> MLADKESLIEALKLALSTEYNVKRNF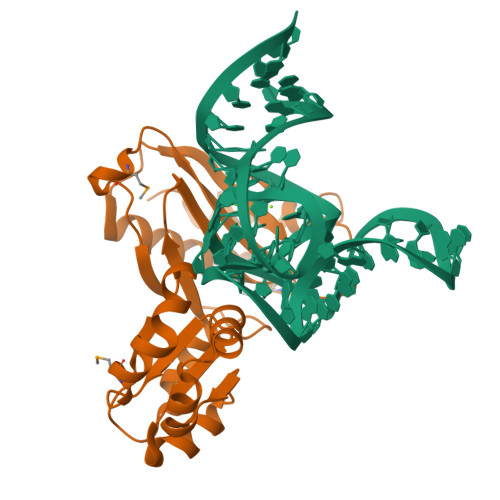TQSVEIILTFKGIDMKKGDLKLREIVPLPKQPSKAKRVLVVPSSEQLEYAKKASPKVVITREELQKLQGQKRPVKKLARQNEWFLINQESMALAGRILGPALGPRGKFPTPLPNTADISEYINRFKRSVLVKTKDQPQVQVFIGTEDMKPEDLAENAIAVLNAIENKAKVETNLRNIYVKTTMGKAVKVKR>MKNELIKRIGIFVCLLIAVNCLSAGNFPVEMRINPSTGAISELTLKGDNRSMNWVVKTDGTQYPWVKDNYGWGLGYFTVVKGRETVKREWRIPVEISPDGMKVLYREGDIRILIKREIKQGDLVEEYSFTNEGEEPVSLYDVAVYTPFNDNYPDAQQCINSRAHTHIWKGGSAAYVNAIRMGDFTPHLGLVVTDGAIRNYEIWERGRKKANSQTRGIIALDLPDLLLKPGESYSLEWHVFAHNGNDDFRHKLLEKGSVLVSCNKYVFEKGEKARVECRSLEPLEACTAKMNGVPVPVKQEGNLCFVEVPMEQAGEVRFDFYYNGNKQTHADCLVISNTADLIRKRVDFIRTRQQMNNPSDLRDGAYMVYDNEGDSIYLNDTPNCNPVDRDEGAERLGMGVLLVKQYLLTKDPELKQSLLRYADFVRRKLQTDNYVTYSSVDQKNRNRGYNYMWVAELYFQMYKVTGDKQFVTDGYKTLKSMFQQFGYGFYAIGIPVRLGLQSLKE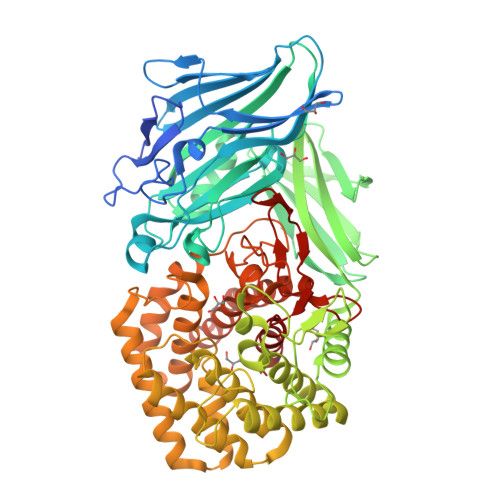AGMKKEYTDLRNDFIKTGDVFVKNGLNYPAHEVNYEQSIVAPAIQFLAQLYLETGSQKYLDEVKRQMPVLEAFNGFQPSYHLNEVAIRHWDGHWFGKRELFGDTFPHYWSTITGAVYYYYALCTGDSSYQKRAENVVRNNLCLFFEDGKASCAYMYPYKIDGVKAEFYDPYANDQDWALVYYLLVNRGL[2x]>[2x]GMETFKQQKVEDFYDIGEELGSGQFAIVKKCREKSTGLEYAAKFIKKRQSRASRRGVCREEIEREVSILRQVLHPNIITLHDVYENRTDVVLILELVSGGELFDFLAQKESLSEEEATSFIKQILDGVNYLHTKKIAHFDLKPENIMLLDKNIPIPHIKLIDFGLAHEIEDGVEFKNIFGTPEFVAPEIVNYEPLGLEADMWSIGVI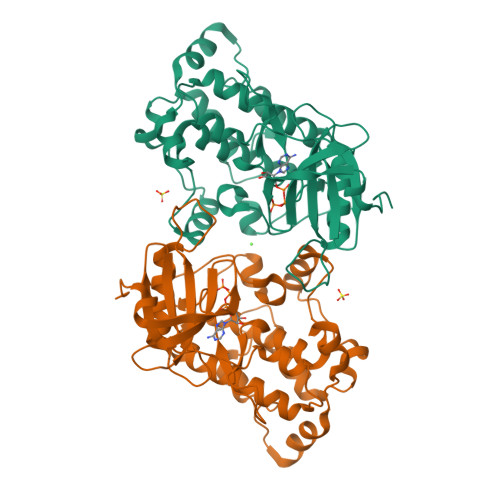TYILLSGASPFLGDTKQETLANITAVSYDFDEEFFSQTSELAKDFIRKLLVKETRKRLTIQEALRHPWITPVDTQQAMVRRESVVNLENFKKQYVRRRWKLSFSIVSLCNHLTRSLMKKVHLRTSEDLRNCESDTEENIARRKALHPRRRSSTS>GGCUCUGGAGAGAACCGUUUAAUCGGUCGCCGAAGGAGCAAGCUCUGCGGAAACGCAGAGUG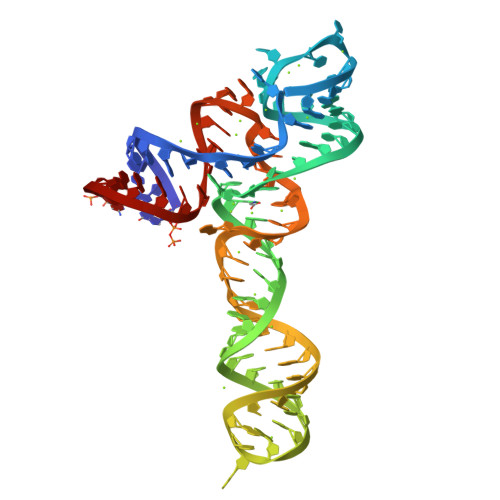AAACUCUCAGGCAAAAGGACAGAGUC[2x]4-(4-METHYLPIPERAZIN-1-YL)-N-[5-(2-THIENYLACETYL)-1,5-DIHYDROPYRROLO[3,4-C]PYRAZOL-3-YL]BENZAMIDE 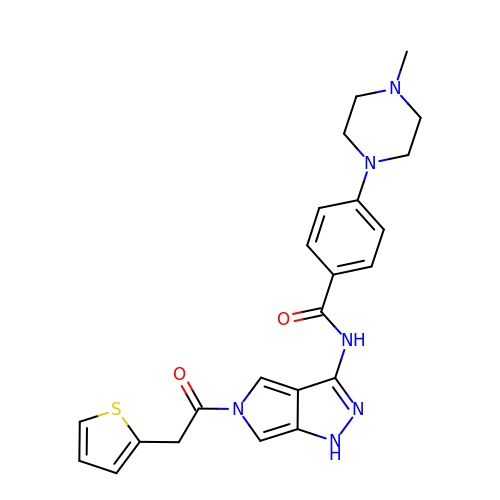| C23 H24 N6 O2 S | TYYNSDQVFIOSFH-UHFFFAOYSA-N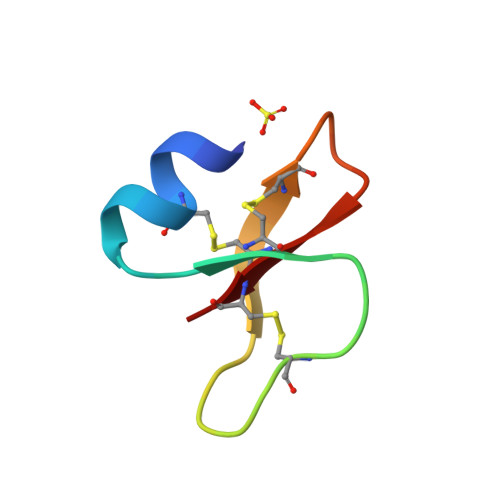>[4x]DHYNCVSAGGQCLYSACPIFTKIQGTCYRGKAKCCK>MGNREQFDLSKYLLEKRKQKGLSQTQVANDTGLSSAYISMLEKGERKRPTQAVIKKLATALSIPNIEMLQIMEYIASMEEDHVKEKDKDTSKQIKLFDLTGLTEASINQIQNQIDQLKSSENNSVIRFFDVTGLSEKDIERVKEEIELLKIRNEYMKLKKD[4x]

Here, we report a structural analog of the oligomerization domain of p53 from the conjugative plasmid pLS20 of the Gram-positive (G+) bacterium Bacillus subtilis. This transcriptional regulator, named Rco, forms tetramers in solution and represses the main conjugation promoter Pc that controls the transcription of genes 28–74. The simultaneous regulation of the Pc and Pr promoters involves RcopLS20-mediated DNA looping, which is achieved through the binding of RcopLS20 to two operators separated by 75 bp and located near the Pc and Pr promoters, each containing multiple direct repeats of the Rco-recognition element (rcoRE; Ramachandran et al., 2014). DNA recognition by Rco is most likely to be achieved through a conserved helix–turn–helix (HTH) domain at its N-terminus, which is followed by a sequence of hitherto unknown function at its C-terminus. Our present results show that the master regulator RcopLS20, which is crucial in the transcriptional regulation of the conjugation operons of plasmid pLS20, contains a tetramerization domain that is likely to be involved in formation of the DNA loop, and that this domain has high structural homology to the tetramerization domain present in the p53 family of tumor repressors.

Crystallization trials on apo full-length (FL) RcopLS20 were not successful, but cocrystallization of FL RcopLS20 with various DNA sequences did result in the formation of crystals. However, structure determination revealed that the crystals contained only part of RcopLS20, corresponding to residues Val125–Lys159 of the FL protein, and no DNA molecules. The asymmetric unit contains four monomers forming one crystallographically independent tetramer. Each monomer consists of an elongated sequence comprising residues Val125–Thr132, which includes a four-amino-acid β-strand formed by residues Arg127–Asp130. This strand is followed by a sharp turn facilitated by the glycine residue Gly133, which is followed by an α-helix comprising residues Glu136–Lys157. The RcoTetpLS20 tetramer consists of a dimer of primary dimers. The primary homodimer is formed by the arrangement of two β-strands from two monomers in an antiparallel fashion and by concomitant antiparallel packing of the helices against one face of the two β-strands.6-[3-(3,3-difluoroazetidin-1-yl)propyl]-4-methylpyridin-2-amine | C12 H17 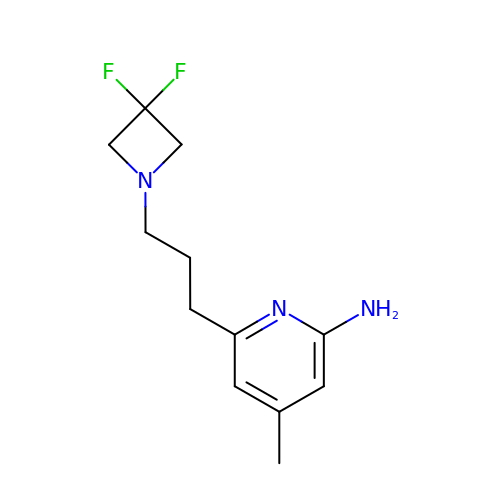F2 N3 | VXUPTLRCBSMECG-UHFFFAOYSA-N> GAMGSGEPQSPSRRVFNPYTEFKEFSRKQIKDMEKMFKQYDAGRDGFIDLMELKLMMEKLGAPQTHLGLKNMIKEVDEDFDSKLSFRAFLLIFRKAAAGELQEDSGLCVLARLSEIDVSS

EFhd2/Swiprosin-1 (EFhd2) is a cytoskeletal Ca2+-binding protein identified in human immune, brain and mast cells. EFhd2 and EFhd1 consist of a disordered N-terminal region followed by two EF-hands and a coiled-coil domain at the C-terminus. We also reported previously that the EF-hands of EFhd2 are involved directly in F-actin bundling in a Ca2+-dependent manner and the coiled-coil domain is essential to the F-actin bundling activity by homodimerisation. Based on the experimental results, we propose that the F-actin bundling activity of EFhd2 depends on structural rigidity conferred by binding of two Ca2+ ions to the EF-hand domains.

We failed to determine the structure of the apo form of EFhd2 owing to structural instability during protein purification; however, we could determine the crystal structures of CDEFhd2 mutants defective for one Ca2+-binding site (E116A for EF1, CDEFhd2EF1; E152A for EF2, CDEFhd2EF2). The overall structures of these two mutants in the presence of Ca2+ are similar to that of Ca2+-bound CDEFhd2 (CDEFhd2EF1, root mean square deviation (RMSD) = 0.34 Å for 102 Cα atoms; CDEFhd2EF2, RMSD = 0.61 Å for 105 Cα atoms), which implies a single Ca2+-loaded EF-hand is sufficient to maintain a stable fold. Although the crystal structures of EF-hand mutants (CDEFhd2EF1 and CDEFhd2EF2) are similar to Ca2+-bound CDEFhd2, we observed structural flexibility in the Ca2+-binding loop of EF1 and the C-terminal linker. Furthermore, comparison of the crystallographic B-factors between Ca2+-bound and EF-hand mutant structures showed that the largest changes in B-factor values were for CDEFhd2EF1 (35.6 Å2), CDEFhd2 (20.4 Å2) and CDEFhd2EF2 (21.5 Å2). To evaluate the effect of Ca2+ on structural dynamics of EFhd2 at the atomic level, we performed ensemble refinement for CDEFhd2, CDEFhd2EF1 and CDEFhd2EF2 using Phenix.ensemble refinement. As expected, Ca2+-bound CDEFhd2 displayed a rigid conformation and CDEFhd2EF1 showed the largest degrees of mobility, indicating that Ca2+ depletion of EF1 has a larger impact on conformational dynamics. In addition, CDEFhd2EF2 also showed a moderate degree of mobility. Interestingly, the C-terminal linker (residues, 176–184) followed by the LM-helix also showed significant RMSF increases in CDEFhd2EF1 and CDEFhd2EF2. Consistent with a previous study showing that thermostability of EFhd2 was restored by Ca2+ at a high temperature, the half aggregation temperature for both EF-hand mutants that bind only one Ca2+ is significantly lower (CDEFhd2EF1: 62.32 ± 0.14 °C, CDEFhd2EF2: 57.90 ± 0.60 °C) than the two Ca2+-bound EFhd2 (CDEFhd2: 84.89 ± 0.01 °C) and is consistent with ref. Even depletion of one Ca2+ site in a two Ca2+-binding protein showed a dramatic reduction in F-actin bundling activity to a level that is similar to that of previously reported data for a two Ca2+-depleted state26.> GDIEQKQAEIIDQLVKRASTCKSEALGPLIIEATSHP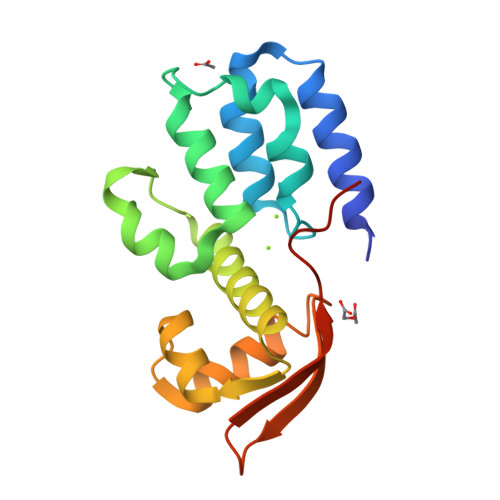SLFAFSEILALPNVAQLEGTTDSVYLDLLRLFAHGTWGDYKCNATRLPHLSPDQILKLKQLTVLTLAESNKVLPYDTLMVELDVSNVRELEDFLINECMYAGIVRGKLDQLKRCFEVPFAAGRDLRPGQLGN> GHMREMLQVERPKLILDDGKRTDGRKPDELRSIKIELGVLKNADGSAIFEMGNTKAIAAVYGPKEMHPRHLSLPDRAVLRVRYHMTPFSTDERKNPAPSRREIELSKVIREALESAVLVELFPRTAIDVFTEILQADA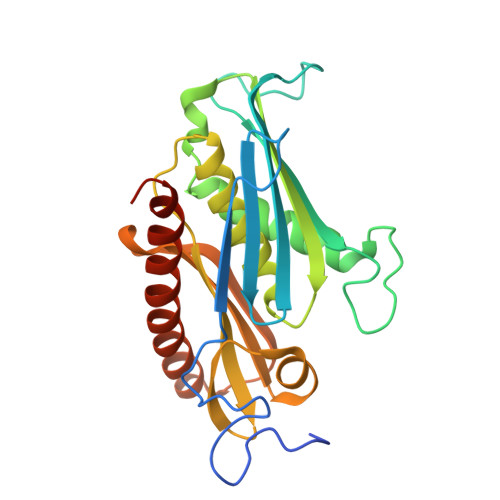GSRLVSLMAASLALADAGIPMRDLIAGVAVGKADGVIILDLNETEAMWGEADMPIAMMPSLNQVTLFQLNGSMTPDEFRQAFDLAVKGINIIYNLEREALKSKYVEFKEEGV>[2x]GPHMEQLEGIMLSPAFQEQMNALMLDPRMLDMMIDQNPQLRNMGPEARQMLRPMFREMMSN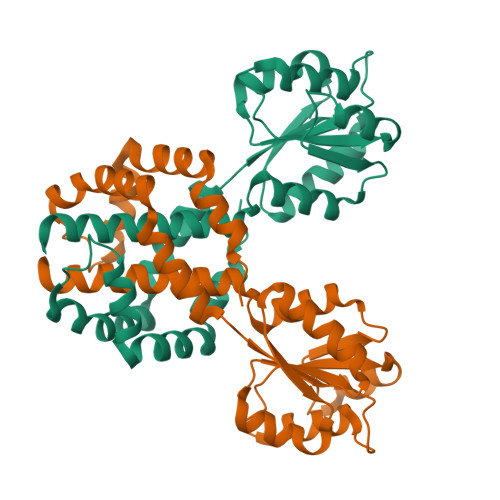PESMRSMMNMGRAWGSKKILIVESDTALSATLRSALEGRGFTVDETTDGKGSVEQIRRDRPDLVVLAVDLSAGQNGYLICGKLKKDDDLKNVPIVIIGNPDGFAQHRKLKAHADEYVAKPVDADQLVERAGALIGFPEGNSMMIALGVACAIALAIAAVYF> DYKDDDDKMTNLPEHQSSPTEQSSAEVKKIPTMIEGFDDISHGGLPQGRTTLVSGTSGTGKTLFAVQ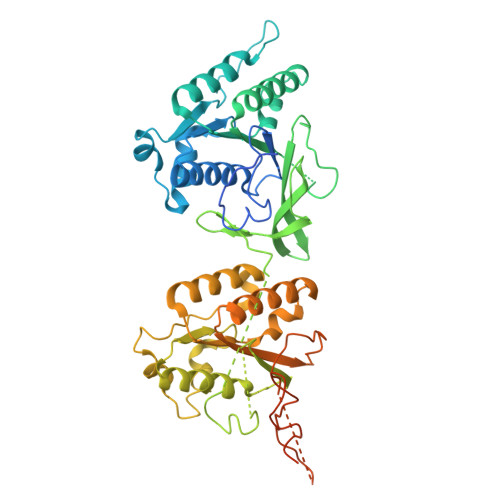FLYNGITIFNEPGIFVTFEESPQDIIKNALSFGWNLQSLIDQGKLFILDASPDPDGQEVAGDFDLSALIERIQYAIRKYKATRVSIDSVTAVFQQYDAASVVRREIFRLAFRLKQLGVTTIMTTERVDEYGPVARFGVEEFVSDNVVILRNVLEGERRRRTVEILKLRGTTHMKGEYPFTINNGINIFPLGAMRLTQRSSNVRVSSGVKTLDEMCGGGFFKDSIILATGATGTGKTLLVSKFLETGCQQGERALLFAYEESRAQLSRNASSWGIDFEELERRGLLRIICAYPESAGLEDHLQIIKSEIADFKPSRVAIDSLSALARGVSNNAFRQFVIGVTGFAKQEEITGFFTNTTDQFMGSNSITESHIETITDTILLLQYVEIRGEMSRAINVFKMRGSWHDKGIREYVITEKGAEIRDSFRNFEGIISGTPTRISVDEKTELARIAKGMQDLESE> SDFYLPGDYLLGGLFSLHANMKGIVHLNFLQVPMCKEYEVKVIGYNLMQAMRFAVEEINNDSSLLPGVLLGYEIVDVCYISNNVQPVLYFLAHEDNLLPIQEDYSNYSSRVVAVIGPDNSESVMTVANFLSLFLLPQITYSAISDELRDKVRFPALLRTTPSADHHIEAMVQLMLHFRWNWIIVLVSNDTYGRDNGQLLGERVARRGICIAFQETLPTLQPNQNMTSEERQRLVTIVDKLQQSTARVVVVFSPDLTLYHFFNEVLRQNFTGAVWIASESWAIDPVLHNLTELRHLGTFLGITIQSVPIPGFSEFREWGPQAGPPPLSRTSQSYTCNQECDNCLNATLSFNTILRLSGERVVYSVYSAVYAVAHALHSLLGCDKSTCTKRVVYPWQLLEEIWKVNFTLLDHQIFFDPQGDVALHLEIVQWQWDRSQNPFQSVASYYPLQRQLKNIQDISWHTINNTIPMSMCSKRCQSGQKKKPVGIHVCCFECIDCLPGTFLNHTEDEYECQA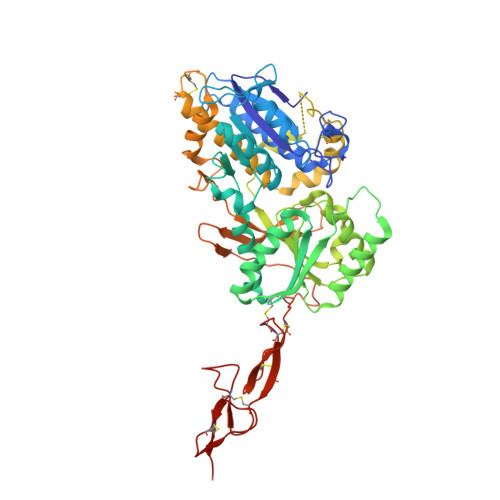CPNNEWSYQSETSCFKRQ> MKRIGILTSGGDAPGMNAAVRAVTRVA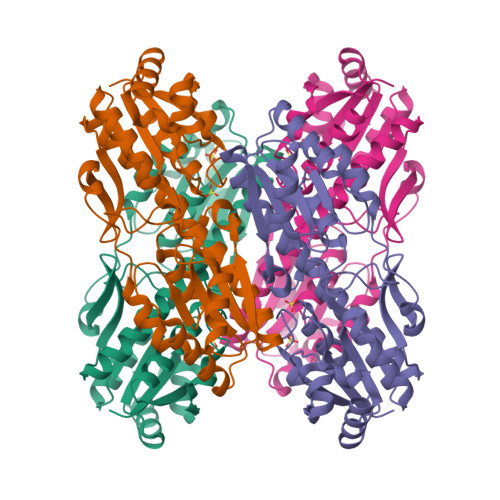IANGLEVFGIRYGFAGLVAGDIFPLESEDVAHLINVSGTFLYSARYPEFAEEEGQLAGIEQLKKHGIDAVVVIGGDGSYHGALQLTRHGFNSIGLPGTIDNDIPYTDATIGYDTACMTAMDAIDKIRDTASSHHRVFIVNVMGRNCGDIAMRVGVACGADAIVIPERPYDVEEIANRLKQAQESGKDHGLVVVAEGVMTADQFMAELKKYGDFDVRANVLGHMQRGGTPTVSDRVLASKLGSEAVHLLLEGKGGLAVGIENGKVTSHDILDLFDESHRGDYDLLKLNADLSR N-(2-phenylethyl)-2-(phenylsulfanyl)-5-sulfamoylpyridine-3-carboxamide 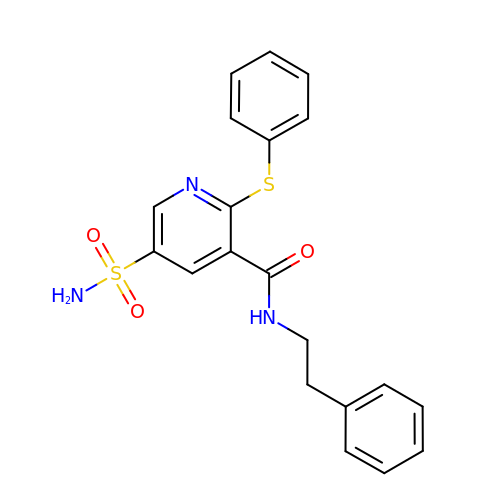| C20 H19 N3 O3 S2 | MGWPMEUXUFQQAQ-UHFFFAOYSA-N> HHHHHHHHVPEAFLLFSRRADIRRISLETNNNNVAIPLTGVKEASALDFDVTDNRIYWTDISLKTISRAFMNGSALEHVVEFGLDYPEGMAVDWLGKNLYWADTGTNRIEVSKLDGQHRQVLVWKDLDSPRALALDPAEGFMYWTEWGGKPKIDRAAMDGSERTTLVPNVGRANGLTIDYAKRRLYWTDLDTNLIESSNMLGLNREVIADDLPHPFGLTQYQDYIYWTDWSRRS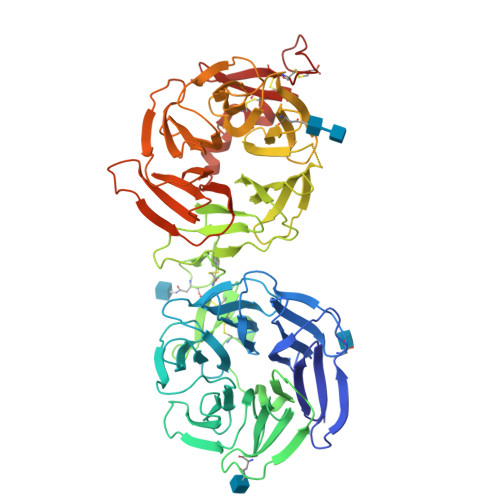IERANKTSGQNRTIIQGHLDYVMDILVFHSSRQSGWNECASSNGHCSHLCLAVPVGGFVCGCPAHYSLNADNRTCSAPTTFLLFSQKSAINRMVIDEQQSPDIILPIHSLRNVRAIDYDPLDKQLYWIDSRQNMIRKAQEDGSQGFTVVVSSVPSQNLEIQPYDLSIDIYSRYIYWTCEATNVINVTRLDGRSVGVVLKGEQDRPRAIVVNPEKGYMYFTNLQERSPKIERAALDGTEREVLFFSGLSKPIALALDSRLGKLFWADSDLRRIESSDLSGANRIVLEDSNILQPVGLTVFENWLYWIDKQQQMIEKIDMTGREGRTKVQARIAQLSDIHAVKELNLQEYRQHPCAQDNGGCSHICLVKGDGTTRCSCPMHLVLLQDELSC> SGGSTWQWVLINISEEARQRIEEYVRRISK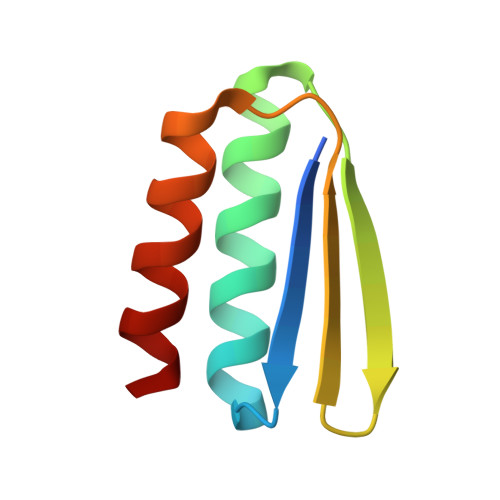KEGTEVHFEKDDGVLHIRVKNLHEKRAREIHEYAKRVIL>MGSSHHHHHHSSGLVPRGSMESGFTSKDTYLSHFNPRDYLEKYYKFGSRHSAESQILKHLLKNLFKIFCLDGVKGDLLIDIGSGPTIYQLLSACESFKEIVVTDYSDQNLQELEKWLKAAPAAFDWSPVVTYVCDLEGNRVKGPEKEEKLRQAVKQVLKCDVTQSQPLGAVPLPPADCVLSTLCLDAACPDLPTYCRAL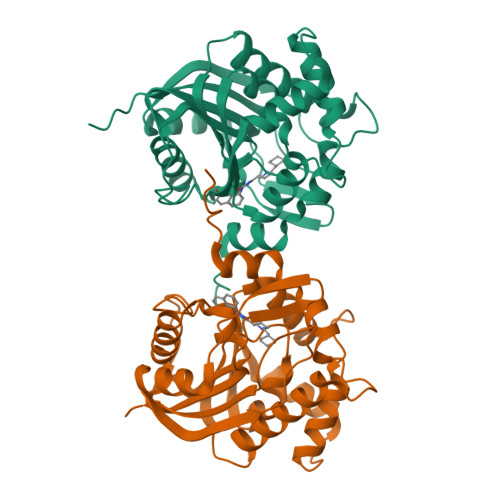RNLGSLLKPGGFLVIMDALKSSYYMIGEQKFSSLPLGREAVEAAVKEAGYTIEWFEVISQSYSSTMANNEGLFSLVARKLSRPL[3x]>ETGYQVRNSSGLYHVTNDCPN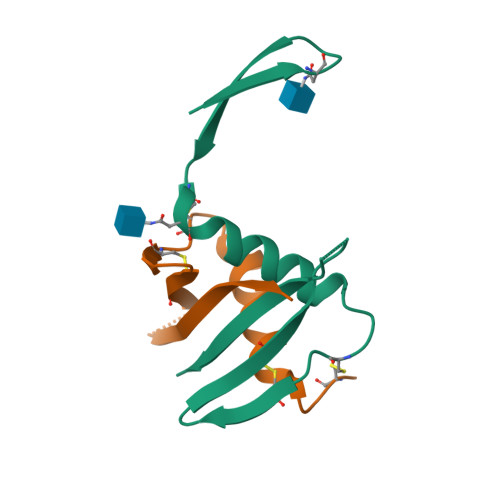SSVVYEAADAILHTPGCVPCVREGQASRCWVAVTPTVATRDGKLPTTQLRRHIDLLVGSATENLYFQ[6x]>[2x]TESPA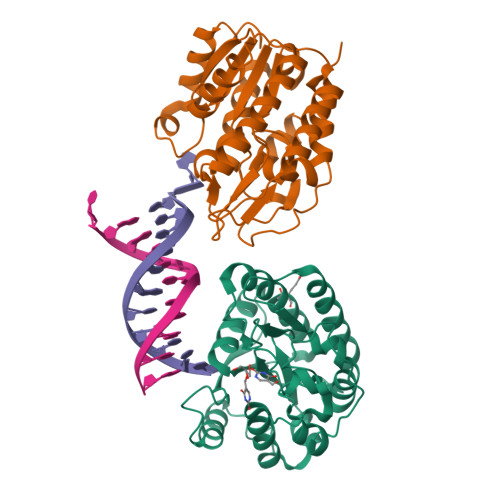DSFLKVELELNLKLSNLVFQDPVQYVYNPLVYAWAPHENYVQTYCKSKKEVLFLGMNPGPFGMAQTGVPFGEVNHVRDWLQIEGPVSKPEVEHPKRRIRGFECPQSEVSGARFWSLFKSLCGQPETFFKHCFVHNHCPLIFMNHSGKNLTPTDLPKAQRDTLLEICDEALCQAVRVLGVKLVIGVGRFSEQRARKALMAEGIDVTVKGIMHPSPRNPQANKGWEGIVRGQLLELGVLSLLTG4-ethyl-6-[5-(1H-pyrazol-4-yl)-1H-pyrrolo[2,3-b]pyridin-3-yl]pyrimidin-2-amine 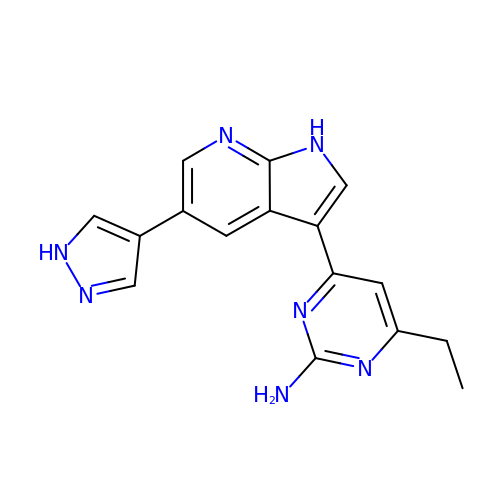| C16 H15 N7 | IVPOFDCEHKLJIL-UHFFFAOYSA-N>MEPHVLGAGLYWLLLPCTLLAASLLRFNALSLVYLLFLLLLPWLPGPSRHSIPGHTGRLLRALLCLSLLFLVAHLAFQICLHTVPHLDQFLGQNGSLWVKVSQHIGVTRLDLKDIFNTTRLVAPDLGVLLASSLCLGLCGRLTRKAGQSRRTQELQDDDDDDDDDDEDIDAAPAVGLKGAPALATKRRLWLASRFRVTAHWLLMTSGRTLVIVLLALAGIAHPSAFSSIYLVVFLAICTWWSCHFPLSPLGFNTLCVMVSCFGAGHLICLYCYQTPFIQDMLPPGNIWARLFGLKNFVDLPNYSSPNALVLNTKHAWPIYVSPGILLLLYYTATSLLKLHKSCPSELRKETPREDEEHELELDHLEPEPQARDATQGEMPMTTEPDLDNCTVHVLTSQSPVRQRPVRPRLAELKEMSPLHGLGHLIMDQSYVCALIAMMVWSIMYHSWLTFVLLLWACLIWTVRSRHQLAMLCSPCILLYGLTLCCLRYVWAMELPELPTTLGPVSLHQLGLEHTRYPCLDLGAMLLYLLTFWLLLRQFVKEKLLKKQKVPAALLEVTVADTEPTQTQTLLRSLGELVTGIYVKYWIYVCAGMFIVVSFAGRLVVYKIVYMFLFLLCLTLFQVYYTLWRKLLRVFWWLVVAYTMLVLIAVYTFQFQDFPTYWRNLTGFTDEQLGDLGLEQFSVSELFSSILIPGFFLLACILQLHYFHRPFMQLTDLEHVPPPGTRHPRWAHRQDAVSEAPLLEHQEEEEVFREDGQSMDGPHQATQVPEGTASKWGLVADRLLDLAASFSAVLTRIQVFVRRLLELHVFKLVALYTVWVALKEVSVMNLLLVVLWAFALPYPRFRPMASCLSTVWTCIIIVCKMLYQLKIVNPHEYSSNCTEPFPNNTNLQPLEINQSLLYRGPVDPANWFGVRKGYPNLGYIQNHLQILLLLVFEAVVYRRQEHYRRQHQQAPLPAQAVCADGTRQRLDQDLLSCLKYFINFFFYKFGLEICFLMAVNVIGQRMNFMVILHGCWLVAILTRRRREAIARLWPNYCLFLTLFLLYQYLLCLGMPPALCIDYPWRWSKAIPMNSALIKWLYLPDFFRAPNSTNLISDFLLLLCASQQWQVFSAERTEEWQRMAGINTDHLEPLRGEPNPIPNFIHCRSYLDMLKVAVFRYLFWLVLVVVFVAGATRISIFGLGYLLACFYLLLFGTTLLQKDTRAQLVLWDCLILYNVTVIISKNMLSLLSCVFVEQMQSNFCWVIQLFSLVCTVKGYYDPKEMMTRDRDCLLPVEEAGIIWDSICFFFLLLQRRIFLSHYFLHVSADLKATALQASRGFALYNAANLKSINFHRQIEEKSLAQLKRQMKRIRAKQEKYRQSQASRGQLQSKDPQDPSQEPGPDSPGGSSPPRRQWWRPWLDHATVIHSGDYFLFESDSEEEEEALPEDPRPAAQSAFQMAYQAWVTNAQTVLRQRRERARQERAEQLASGGDLNPDVEPVDVPEDEMAGRSHMMQRVLSTMQFLWVLGQATVDGLTRWLRAFTKHHRTMSDVLCAERYLLTQELLRVGEVRRGVLDQ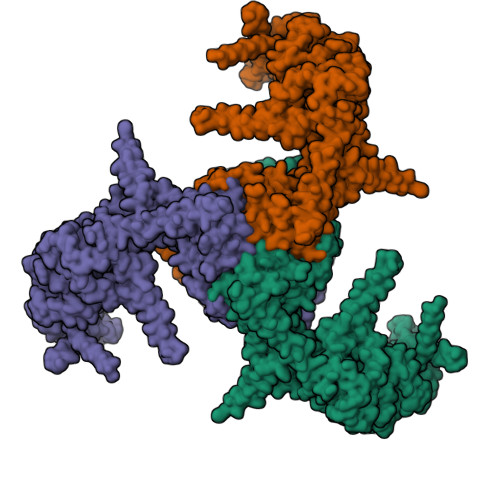LYVGEDEATLSGPVETRDGPSTASSGLGAEEPLSSMTDDTSSPLSTGYNTRSGSEEIVTDAGDLQAGTSLHGSQELLANARTRMRTASELLLDRRLHIPELEEAERFEAQQGRTLRLLRAGYQCVAAHSELLCYFIIILNHMVTASAASLVLPVLVFLWAMLTIPRPSKRFWMTAIVFTEVMVVTKYLFQFGFFPWNSYVVLRRYENKPYFPPRILGLEKTDSYIKYDLVQLMALFFHRSQLLCYGLWDHEEDRYPKDHCRSSVKDREAKEEPEAKLESQSETGTGHPKEPVLAGTPRDHIQGKGSIRSKDVIQDPPEDLKPRHTRHISIRFRRRKETPGPKGTAVMETEHEEGEGKETTERKRPRHTQEKSKFRERMKAAGRRLQSFCVSLAQSFYQPLQRFFHDILHTKYRAATDVYALMFLADIVDIIIIIFGFWAFGKHSAATDIASSLSDDQVPQAFLFMLLVQFGTMVIDRALYLRKTVLGKLAFQVVLVVAIHIWMFFILPAVTERMFSQNAVAQLWYFVKCIYFALSAYQIRCGYPTRILGNFLTKKYNHLNLFLFQGFRLVPFLVELRAVMDWVWTDTTLSLSNWMCVEDIYANIFIIKCSRETEKKYPQPKGQKKKKIVKYGMGGLIILFLIAIIWFPLLFMSLIRSVVGVVNQPIDVTVTLKLGGYEPLFTMSAQQPSIVPFTPQAYEELSQQFDPYPLAMQFISQYSPEDIVTAQIEGSSGALWRISPPSRAQMKQELYNGTADITLRFTWNFQRDLAKGGTVEYTNEKHTLELAPNSTARRQLAQLLEGRPDQSVVIPHLFPKYIRAPNGPEANPVKQLQPDEEEDYLGVRIQLRREQVGTGASGEQAGTKASDFLEWWVIELQDCKADCNLLPMVIFSDKVSPPSLGFLAGYGIVGLYVSIVLVVGKFVRGFFSEISHSIMFEELPCVDRILKLCQDIFLVRETRELELEEELYAKLIFLYRSPETMIKWTRERE[3x]> SMKLSSSEKEKLLKKLKALGAKEEKPPEHAQYRLRLNDAILTVYKSGSVVYGGKGREKLKELVAETVLSDTELPRIGCNEAGKGEFVGPLVVACIVADEKCLKRLIELGVKDSKKLSNEKVEELASEITETCHGKVKLLIPEKYNRAYSKFKNINRLLEAVYREIVSDLCEKFSPKVVVVDKFSNRAEEVLKDVVKGARLEVRPKAEDDLAVAAASIVAK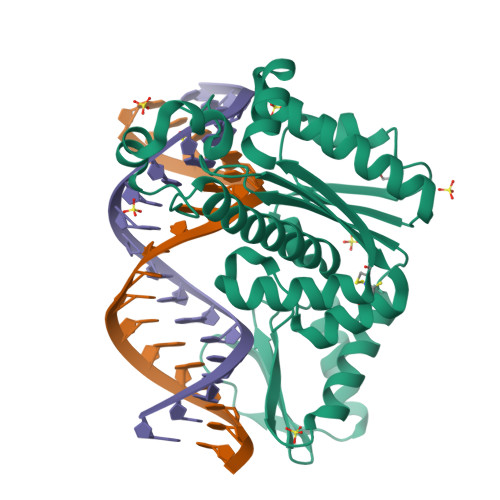AVRLKTMKELEKRFKVKLPEGNTGLAELLKKTPKELHEKLFKLHFSVGGKK> MLGEDEGNTVLEKGNNPSVKQGEVGAVFIVPKILIREHERVILKQILQILDQDELVQPPLDKFPYKKLELPKYIDELKTRDATNTSYKMIQLDAYGEKKVGSNGELFGGRHYLFNTFTFTAHMGVLLVLLQDVIKVLYQSNATHDEDEFIVQHDQILVMETSEEQTKFLAKNGVIPEESKGSFKYITARSAFVEFGASVIAGGQRIVDDYWESLAKKQNLSSHQRVFKLSTNLISKISLLRPSFQNNRISNANEISANTNNTCTISTSKFESQYPIVTEQPSAEIREAYIENFAKGEHISAIVPGQSISGTLELSAQFRVPRYHSKNSFQQALQMKAMDIPIGRHEELLAQYESQAPDGSASISLPNHIPSVNPSNKPIKRMLSSILDINVSSSKNKKSEENEMIKPMNKGQHKNNTSLNINGWKFESLPLKSAENSGKQQYYRGLPLYEKNTLLERLKQLTPNEIKELEHLHDAVFVNTGLQNVRKVRTKKWKKYWQYKAGIPIGLKRSQLDEFKNKYLKDVLAQTSVTTNFNEITNTDETITTKRVPNPNFLGNCNIKDFKPPYIYSHVNKVPQNVAGDKTAVKLDTEVKNTNANPVVATDPVAAKP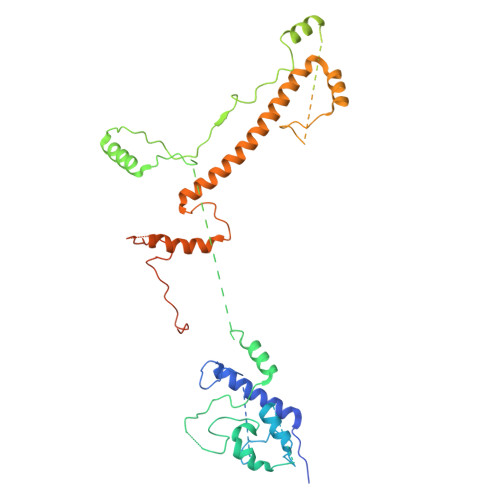DNLANFSNEVAMNN> MASWSHPQFEKGGENNSLAPLRVGILGFGGLGQAAARLLA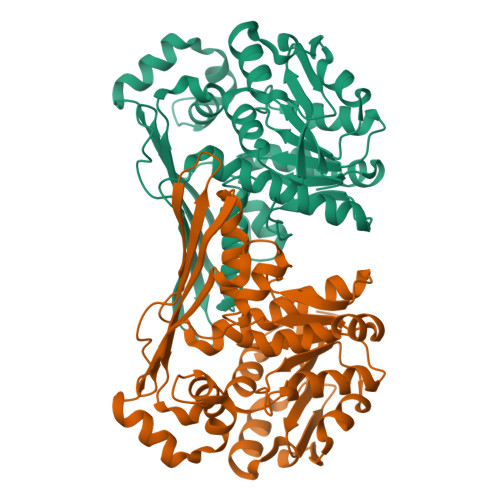PKQEMKLVAVADRHGYLYDADGIDVDNAVQAYTQQGSVGKAKKGQMSEQSIEDLIGEGEVDGYFLALPNLPNTFMADVTRQFIASGWQGVLVDALKRTSAVEQLITLREDLAQAGITYMTGCGATPGLLTAAAAIASQSFQEIHQVKITFGVGIANWEAYRATIREDIAHMPGYNVDKAQAMTDAEVAALLDQTNGILALEDMEHADDIMLELAGICHRDQVTVGGVVDTRNPKKPLSTHVKITGRTFEGKISSHTFTLGDETSMAANVCGPAFGYLKAGYGLHRQGLKGLFTAADVMPKFVR> GKNAPSTAGLGYGSWEIDPKDLTFLKELGTGQFGVVKYGKWRGQYDVAIKMIKEGSMSEDEFIEEAKVMMNLSHEKL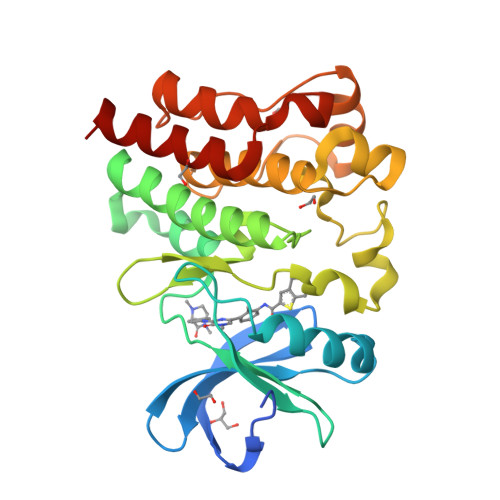VQLYGVCTKQRPIFIITEYMANGCLLNYLREMRHRFQTQQLLEMCKDVCEAMEYLESKQFLHRDLAARNCLVNDQGVVKVSDFGLSRYVLDDEYTSSVGSKFPVRWSPPEVLMYSKFSSKSDIWAFGVLMWEIYSLGKMPYERFTNSETAEHIAQGLRLYRPHLASEKVYTIMYSCWHEKADERPTFKILLSNILDVMDEES>[2x]SRHSEKIAIRDFQ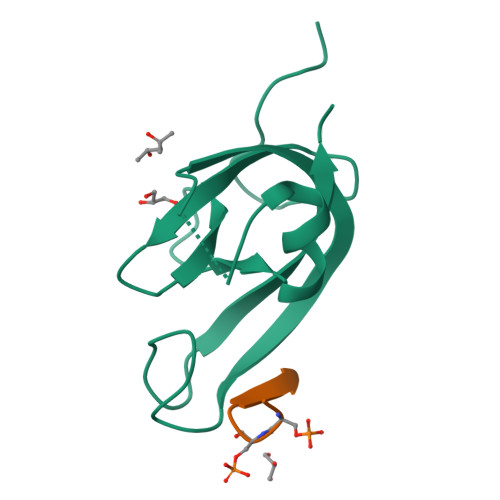VGDLVLIILDERHDNYVLFTVSPTLYFLHSESLPALDLKPGEGASGASRRPWVLGKVMEKEYCQAKKAQNRFKVPLGTKFYRVKAVSWNKKV;>[2x]SSGTSSEFEVV> XPPG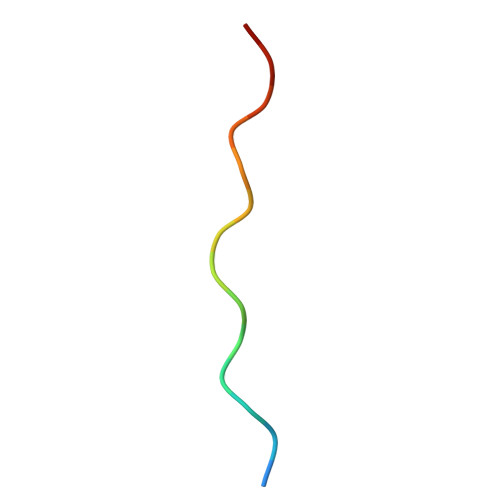PPGPRGPPGPPX> MEPIHILITGAAGQIGYALTFRIAKGDLCGDRKVVLHLLEIPFGMKALEGCVMELQDCAFPNVAGIVWTDKVEEAFKGVDVAFLVGSFPRKDGMDRSDLLAKNGGIFTVQGKALNDYAKPTVKVLVVGNPANTNCLIAQASAPKLQNKNWCAMTRLDHNRMVGALAAKFGVTPEKIHKVCIWGNHSNTQVPDTTHATVDLPEGTVKVADKLPKEYLEGEFAQMIATRGGAVIKMRGASSAASA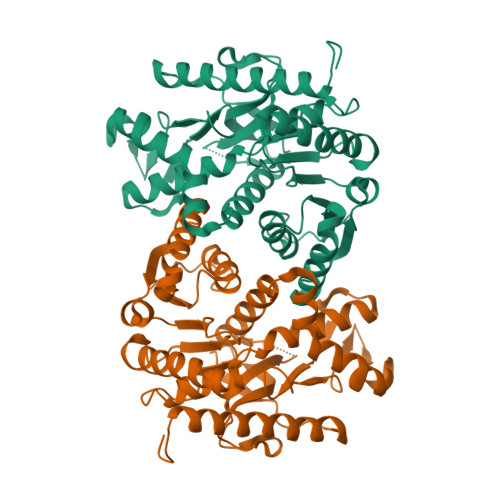ANAALTCVKDWLYGTAEGDFVSMAIPVPDNEPYGIKQGTIFSFPVTVSKDGEVHVVEGLELNDWVKGRLEATEKELIGEKETAWKVLGLLEHHHHHH>[2x]AKPLTDQEKRRQISIRGIVGVENVAELKKSFNRHLHFTLVKDRNVATTRDYYFALAHTVRDHLVGR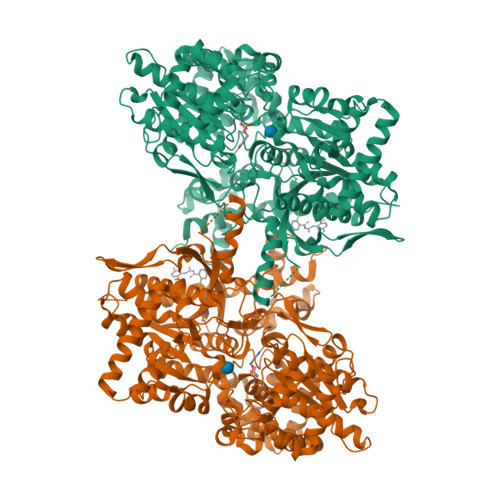WIRTQQHYYDKCPKRVYYLSLEFYMGRTLQNTMINLGLQNACDEAIYQLGLDIEELEEIEEDAGLGNGGLGRLAACFLDSMATLGLAAYGYGIRYEYGIFNQKIRDGWQVEEADDWLRYGNPWEKSRPEFMLPVHFYGKVEHTNTGTKWIDTQVVLALPYDTPVPGYMNNTVNTMRLWSARAPNDFNLRDFNVGDYIQAVLDRNLAENISRVLYPNDNFFEGKELRLKQEYFVVAATLQDIIRRFKASKFGSTRGAGTVFDAFPDQVAIQLNDTHPALAIPELMRIFVDIEKLPWSKAWELTQKTFAYTNHTVLPEALERWPVDLVEKLLPRHLEIIYEINQKHLDRIVALFPKDVDRLRRMSLIEEEGSKRINMAHLCIVGSHAVNGVAKIHSDIVKTKVFKDFSELEPDKFQNKTNGITPRRWLLLCNPGLAELIAEKIGEDYVKDLSQLTKLHSFLGDDVFLRELAKVKQENKLKFSQFLETEYKVKINPSSMFDVQVKRIHEYKRQLLNCLHVITMYNRIKKDPKKLFVPRTVIIGGKAAPGYHMAKMIIKLITSVADVVNNDPMVGSKLKVIFLENYRVSLAEKVIPATDLSEQISTAGTEASGTGNMKFMLNGALTIGTMDGANVEMAEEAGEENLFIFGMRIDDVAALDKKGYEAKEYYEALPELKLVIDQIDNGFFSPKQPDLFKDIINMLFYHDRFKVFADYEAYVKCQDKVSQLYMNPKAWNTMVLKNIAASGKFSSDRTIKEYAQNIWNVEPSDLKISLSNESNKVNGN>MDAKKVAKKAADQAANRIRELAQVLVELLKEALKLDLTQEMRKKLIERYAAAIIRAIGDINNAIYQAKQEAEKLKKAGLVDSDQLDALLRALDELQKVASKAANQLGRLFEEALKRLDKDNGGEEEKDRTAKWFEFEARAIAIALTLAAIGDVFDLEKEWRKLK[2x];>[4x]GHMMSQSNRELVVDFLSYKLSQK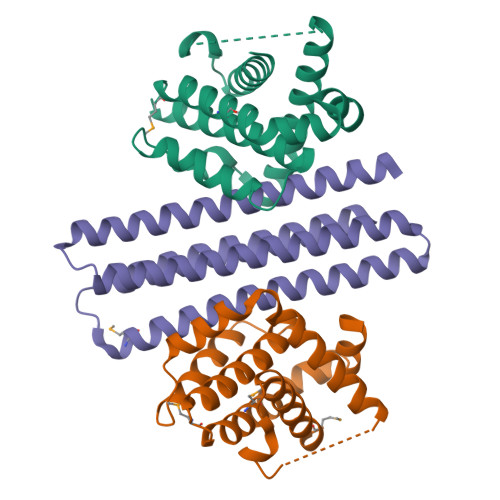GYSWSQFSDVEENRTEAPEGTESEAVKQALREAGDEFELRYRRAFSDLTSQLHITPGTAYQSFEQVVNELFRDGVNWGRIVAFFSFGGALCVESVDKEMQVLVSRIAAWMATYLNDHLEPWIQENGGWDTFVELYGNNAAAESRKGQER> T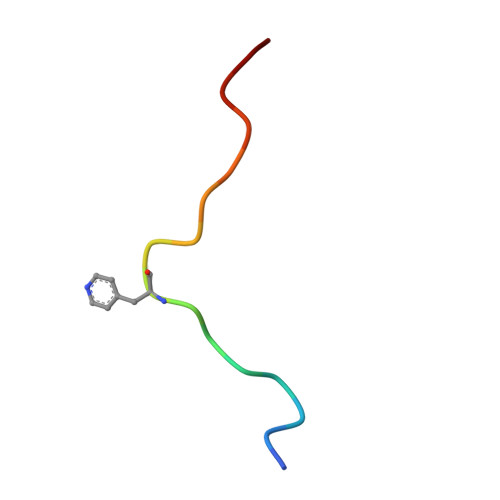LKYPIEXGIVTNWDD> MPFPFGKSHKSPADIVKNLKESMAVLEKQDISDKKAEKATEEVSKNLVAMKEILYGTNEKEPQ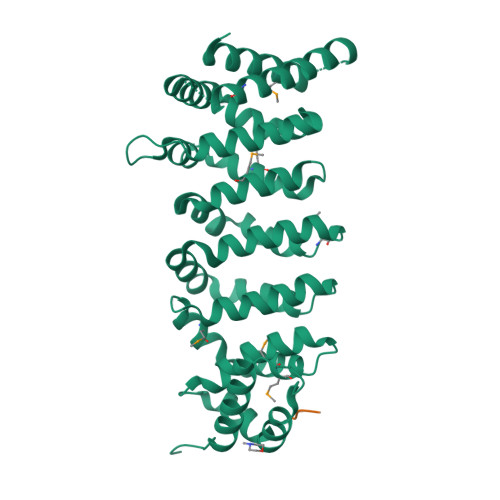TEAVAQLAQELYNSGLLSTLVADLQLIDFEGKKDVAQIFNNILRRQIGTRTPTVEYICTQQNILFMLLKGYESPEIALNCGIMLRECIRHEPLAKIILWSEQFYDFFRYVEMSTFDIASDAFATFKDLLTRHKLLSAEFLEQHYDRFFSEYEKLLHSENYVTKRQSLKLLGELLLDRHNFTIMTKYISKPENLKLMMNLLRDKSRNIQFEAFHVFKVFVANPNKTQPILDILLKNQAKLIEFLSKFQNDRTEDEQFNDEKTYLVKQIRDLKRPAQQEA;> NLEELEVDDWEF>[8x]QTVARKCSLTGEWDNDLGSIMTIGAVNDNGEFDGTYITAVADNPGNITLSPLLGIQHKRAS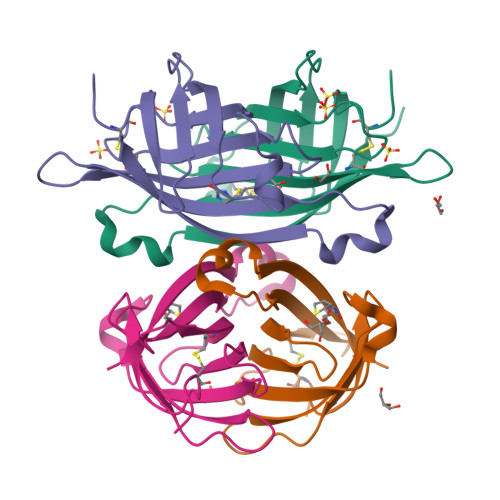QPTFGFTVHWNFSESTSVFVGQCFVDRSGKEVLKTKWLQRLAVDDISDDWIATRVGNNDFTRQHTVEE> GSAKDPSLPERIDTFTELFNYQLAEKSYDIRVLQSNYPTKLLSPDSMLPQTADYPLKDIQQLYQLANTCRGKLPLSPLITEPLVFTRAICKGTQLTPRWFSRSGLIHPGGGSYAARYVDKYPELQDKLAQYMHIKERKNVQGDELLASLKSMNDDAINALIAGASMFIEQNELWLRRGDHYFVFPKSVWQENVANAGLSFKLASQTKSCFVKRG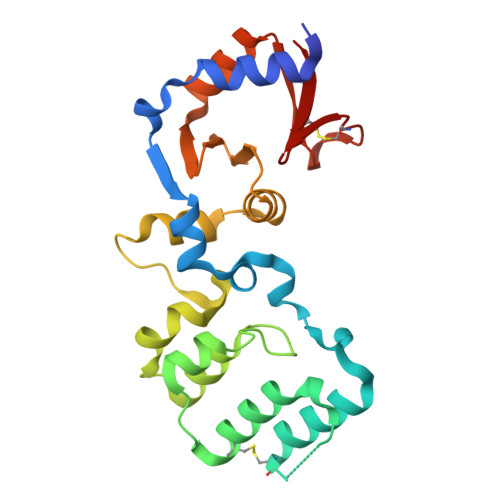NICWDVE> SNAADKITVFAAASLTNALQDIAVQYKQEKQVDVVASYASSSTLARQIEQGAPADLFISADQQWMDYAIDKQQIVANTRYTLLGNELVLIAPQDSQIDKVEIDKKTDWKKLLEGGRLAVGDPDHVPAGIYAKESLENLGAWSTLAPEMARANNVRSAMALVERAEAPLGIVYGSDAVASKKVKVVGIFPE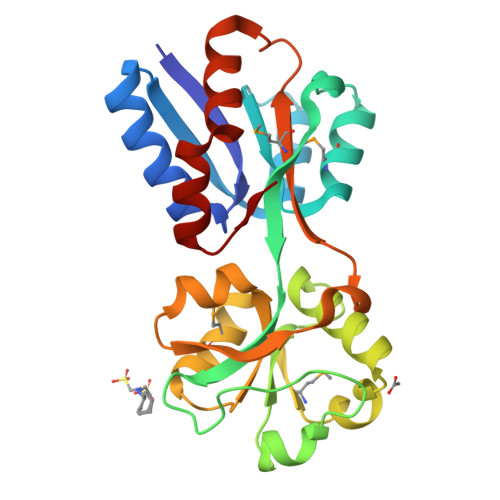ASHKPVEYPMAIVKGHDNPTVTAFYDYLKSPAAAVIFKNYGFTPR> LTDSVYERLLSERIIFLGSEVNDEIANRLCAQILLLAAEDASKDISLYINSPGGSISAGMAIYDTMVLAPCDIATYAMGMAASMGEFLLAAGTKGKRYALPHARILMHQPLGGVTGSAADIAIQAEQFAVIKKEMF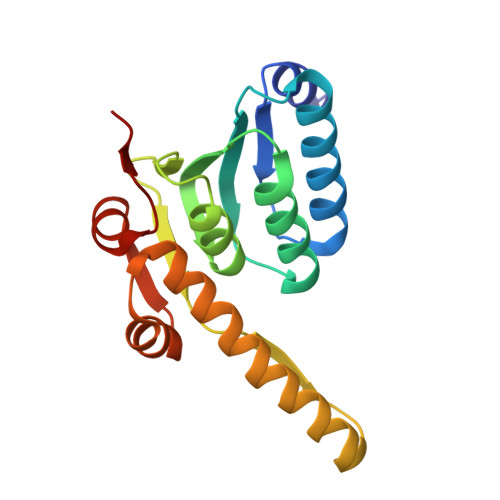RLNAEFTGQPIERIEADSDRDRWFTAAEALEYGFVDHIITR>AEGTRGRSSTARCSLFGSDFVNTFDGSMYSFAGYCSYLLAGGCQKRSFSIIGDFQNGKRVSLSVYLGEFFDIHLFVNGTVTQGDQRVSMPYASKGLYLETEAGYYKLSGEAYGFVARIDGSGNFQVLLSDRYFNKTCGLCGNFNIFAEDDFMTQEGTLTSDPYDFANSWALSSGEQWCERASPPSSSCNISSGEMQKGLWEQCQLLKSTSVFARCHPLVDPEPFVALCEKTLCECAGGLECACPALLEYARTCAQEGMVLYGWTDHSACSPVCPAGMEYRQCVSPCARTCQSLHINEMCQERCVDGCSCPEGQLLDEGLCVESTECPCVHSGKRYPPGTSLSRDCNTCICRNSQWICSNEECPGECLVTGQSHFKSFDNRYFTFSGICQYLLARDCQDHSFSIVIETVQCADDRDAVCTRSVTVRLPGLHNSLVKLKHGAGVAMDGQDVQLPLLKGDLRIQHTVTASVRLSYGEDLQMDWDGRGRLLVKLSPVYAGKTCGLCGNYNGNQGDDFLTPSGLAEPRVEDFGNAWKLHGDCQDLQKQHSDPCALNPRMTRFSEEACAVLTSPTFEACHRAVSPLPYLRNCRYDVCSCSDGRECLCGALASYAAACAGRGVRVAWREPGRCELNCPKGQVYLQCGTPCNLTCRSLSYPDEECNEACLEGCFCPPGLYMDERGDCVPKAQCPCYYDGEIFQPEDIFSDHHTMCYCEDGFMHCTMSGVPGSLLPDAVLSSPLSHRSKR[4x];>[4x]SLSCRPPMVKLVCPADNLRAEGLECTKTCQNYDLECMSMGCVSGCLCPPGMVRHENRCVALERCPCFHQGKEYAPGETVKIGCNTCVCQDRKWNCTDHVCDATCSTIGMAHYLTFDGLKYLFPGECQYVLVQDYCGSNPGTFRILVGNKGCSHPSVKCKKRVTILVEGGEIELFDGEVNVKRPMKDETHFEVVESGRYIILLLGKALSVVWDRHLSISVVLKQTYQEKVCGLCGNFDGIQNNDLTSSNLQVEEDPVDFGN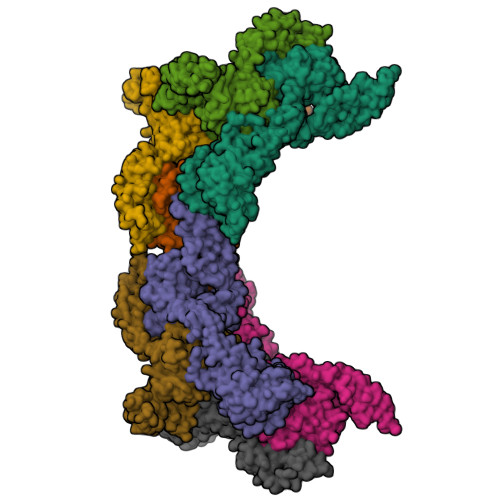SWKVSSQCADTRKVPLDSSPATCHNNIMKQTMVDSSCRILTSDVFQDCNKLVDPEPYLDVCIYDTCSCESIGDCACFCDTIAAYAHVCAQHGKVVTWRTATLCPQSCEERNLRENGYECEWRYNSCAPACQVTCQHPEPLACPVQCVEGCHAHCPPGKILDELLQTCVDPEDCPVCEVAGRRFASGKKVTLNPSDPEHCQICHCDVVNLTCEACQEPGGLVVPPHHHHHH>GAASRLRSPSVLEVREKGYERLKEELAKAQRELKLKDEECERLSKVRDQLGQELEELTASLFEEAHKMVREANIKQATAEKQLKEAQGKIDVLQAEVAALKTLVLS[3x];> GASSRLRSPSVLEVREKGYERLKEELAKAQRELKLKDEECERLSKVRDQLGQELEELTASLFEEAHKMVREANIKQATAEKQLKEAQGKIDVLQAEVAALKTLV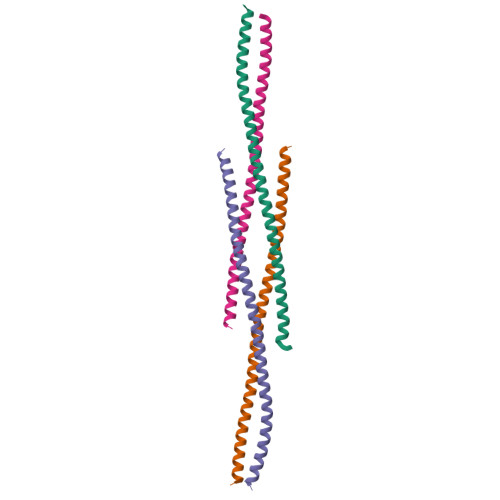LS>[2x]GSSGSSGMANERMNLMNMAKLSIKGLIESALNLGRTLDSDYAPLQQFFVVMEHCLKHGLKAKKTFL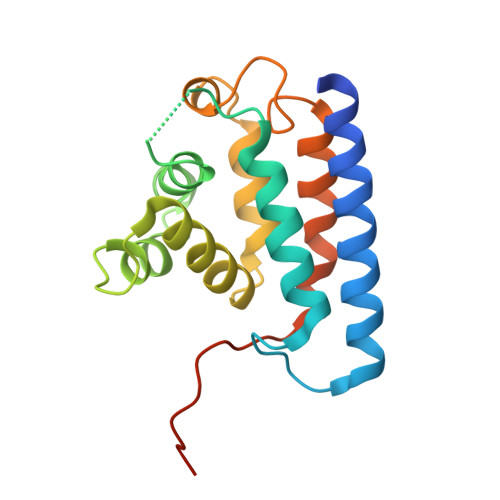GQNKSFWGPLELVEKLVPEAAEITASVKDLPGLKTPVGRGRAWLRLALMQKKLSEYMKALINKKELLSEFYEVNALMMEEEGAIIAGLLVGLNVIDANFCMKGEDLDSQVGVID> QSTRVEEGSKVAISCSLMADEGVHWFRQGKKPNPEFLVYISGIGSQNPAAKDKYSADKSSQKVTLTVKDFRKEDSGKYYCLMVKNRALTFGKPQDYYVEE

The CD8 molecule is a type I membrane glycoprotein with two isoforms, CD8α and CD8β, which can form homodimeric (CD8αα) or heterodimeric (CD8αβ) complexes. To ensure efficient T cell activation, CD8 acts as a co-receptor to stabilize the interaction of TCR with MHC I on the surface of antigen-presenting cells (APCs). In this study, CD8α and CD8β orthologues (termed ScCD8α and ScCD8β) were identified in small-spotted catshark (Scyliorhinus canicula).

The structure of recombinant ScCD8α extracellular region was solved at a resolution of 1.35 Å with a space group of C121 and further refined to a Rwork/Rfree factor of 0.198/0.2. The structure is composed of two molecules arranged in the asymmetric unit. Despite low sequence homology with known CD8α molecules, ScCD8αα retains typical IgSF V architecture. Like its counterparts in higher vertebrates, the ScCD8α dimer consists of 2 anti-parallel β sheets containing 10 β strands, labeled as A, A’, B, C, C’, D, E, F, G, G’. Notably, the A strand is in the back β sheet, lying parallel to strand G’, an arrangement seen only in grass carp CD8α thus far. Two cysteines (Cys19 and Cys84) form a disulphide bond linking the front and back sheet of ScCD8α and stabilizing the IgSF V architecture. The ScCD8αα interface contains four inter-chain hydrogen bonds, which are formed by Gln32 (chain A) and Tyr83 (chain B), Asn51 (chain A) and Arg90 (chain B), Gln32 (chain B) and Tyr83 (chain A), Asn51 (chain B) and Arg90 (chain A), respectively. Five aromatic residues including Phe30 (strand B), Phe40 and Tyr43 (strand C), Tyr83 (strand F) and Phe94 (strand G) are located in the center of ScCD8αα dimer, forming a hydrophobic core with a BSA of 315.51 Å2 and contributing to 58.2% of the total hydrophobic force. The structure of ScCD8αα shows a canonical cavity is formed between the CDR loops of the two monomers. Structure alignment showed that His28ScCD8α is placed approximately 1.2Å away from the surface, which may explain the formation of the cavity.>MNLTGKTALVTGSTSGIGLGIAQVLAQAGATLILNGFGDVDAAKDAVAQYGKTPGYHGADLSDEAQIADMMRYAESEFGGVDILINNAGIQHVSPIETFPVDKWNAIIAINLSSVFHTTRLALPGMRARNWGRIINIASVHGLVASKEKSAYVAAKHGVVGLTKTIALETAQT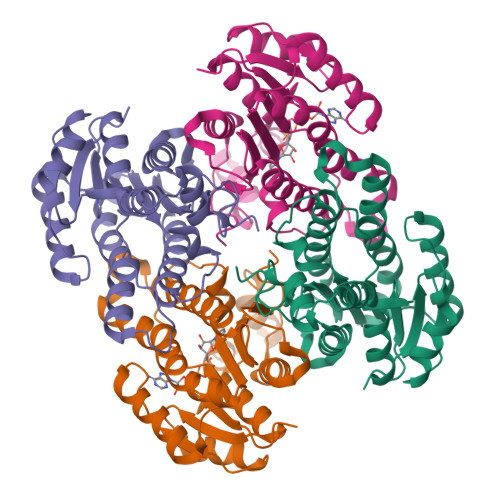EITCNALCPGWVLTPLVQQQIDKRIAEGAEPEAARDALLAEKQPSREFVTPEQLGNLALFLCSDGAAQVRGVAWNMDGGWVAQ[4x]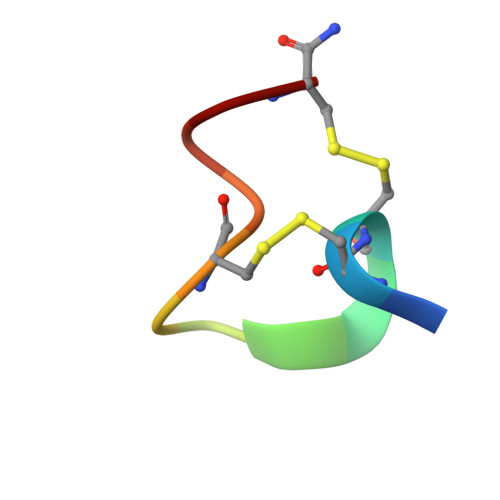> GCCSDPRCAWRC>MEGNGSQLGSRQHQESQAAVDPPGATGPTTSHVVVSNPEQPNGPAQRLEMAVATGAIQSNVPEAIRNCFAVYRTFAWNDRMPAGTFLGSVSLHPNINPYTSHLSGMWAGWGGSFESRVSISGSGVFAGRVVASVIPPGVDPSSIRDPGVLPHAFVDARITEPVSFMIPDVRNTDYHRMDGNEPTCSLGLWVYQPLINPFSTSAVSTCWVSIETKPGGDFDFCLLKPPGQRMENGVSPEGLLPRRLGYARGNRVGGLVVGLVLVADHHQVNRHFNANSITYGWSTAPVNPMAAEIVVKHDYTNNRNAWLSIGAKNKGPLFPGLPNHFPDSCASTLVGAMDTGRHMPATGVCGPAIGFQDNGDVFENETPAVMFATFNPLTGGDNTNPIALYDSINPASLAVMCTKSNSNFDSSGFANDKNVVVQMSWEMYTNSQQIQGRVTPMQGTNFVFTSSGAN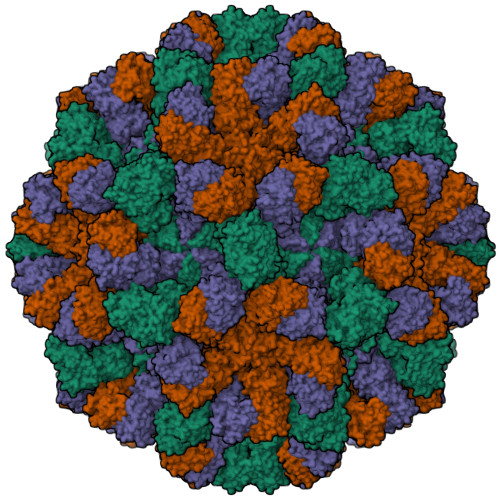TLALWEERLLSYDGHQAILYSSQMERTSEYFQNDNVNIPPGSMAVFNVETNSASFQIGIREDGYMVTGGTIGTHVVLDPETRFQYVGLLPLTAALAGPNGNSGRARRVFQ[3x]> MGSVTPIPLPKIDEPEEYNTNYILFWNHVGLELNRVTHTVGGPLTGPPLSARALGMLHLAIHDAYFSICPPTDFTTFLSPDTENAAYRLPSPNGANDARQAVAGAALKMLSSLYMKPVEQPNPNPGANISDNAYAQLGLVLDRSVLEAPGGVDRESASF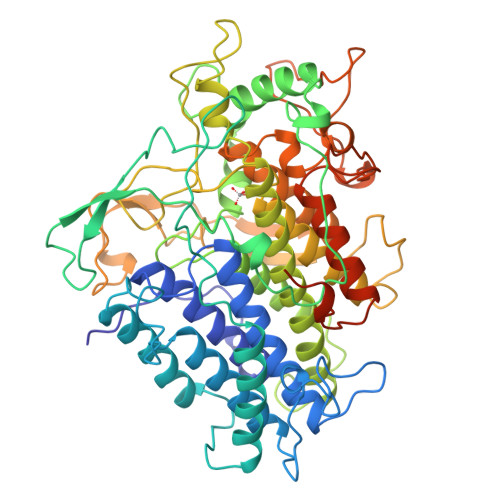MFGEDVADVFFALLNDPRGASQEGYHPTPGRYKFDDEPTHPVVLIPVDPNNPNGPKMPFRQYHAPFYGKTTKRFATQSEHFLADPPGLRSNADETAEYDDAVRVAIAMGGAQALNSTKRSPWQTAQGLYWAYDGSNLIGTPPRFYNQIVRRIAVTYKKEEDLANSEVNNADFARLFALVDVACTDAGIFSWKEKWEFEFWRPLSGVRDDGRPDHGDPFWLTLGAPATNTNDIPFKPPFPAYPSGHATFGGAVFQMVRRYYNGRVGTWKDDEPDNIAIDMMISEELNGVNRDLRQPYDPTAPIEDQPGIVRTRIVRHFDSAWELMFENAISRIFLGVAWRFDAAAARDILIPTTTKDVYAVDNNGATVFQNVEDIRYTTRGTREDEEGLFPIGGVPLGIEIADEIFNNGLKPTPPEIQPMPQETPVQKPVGQQPVKGMWEEEQAPVVKEAP1,4:3,6-dianhydro-2-O-(6-chloro-5-{4-[1-(hydroxymethyl)cyclopropyl]phenyl}-1H-benzimidazol-2-yl)-D-mannitol 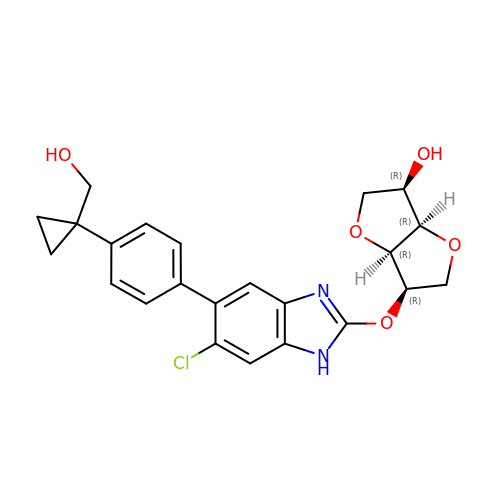| C23 H23 Cl N2 O5 | IMVYDTHPRTUISR-XRXFAXGQSA-N>MAASTPVVVDIHTHMYPPSYIAMLEKRQTIPLVRTFPQADEPRLILLSSELAALDAALADPAAKLPGRPLSTHFASLAQKMHFMDTNGIRVSVISLANPWFDFLAPDEAPGIADAVNAEFSDMCAQHVGRLFFFAALPLSAPVDAVKASIERVKNLKYCRGIILGTSGLGKGLDDPHLLPVFEAVADAKLLVFLHPHYGLPNEVYGPRSEEYGHVLPLALGFPMETTIAVARMYMAGVFDHVRNLQMLLAHSGGTLPFLAGRIESCIVHDGHLVKTGKVPKDRRTIWTVLKEQIYLDAVIYSEVGLQAAIASSGADRLMFGTNH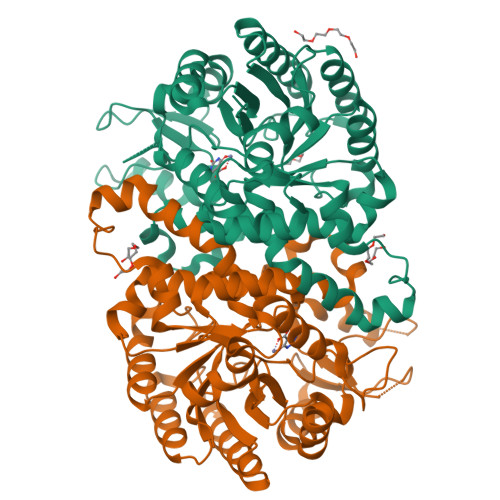PFFPPIEEDVQGPWDSSRLNAQAVIKAVGEGSSDAAAVMGLNAVRVLSLKAE[2x]>GPLGSISQNKRRYRKDGFDLDLTYVTDHVIAMSFPSSGRQSLFRNPIGEVSRFFKTKHPDK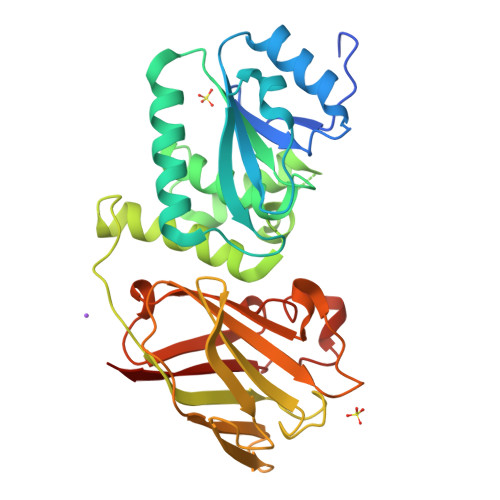FRIYNLCSERGYDETKFDNHVYRVMIDDHNVPTLVDLLKFIDDAKVWMTSDPDHVIAIHCKGGKGRTGTLVSSWLLEDGKFDTAKEALEYFGSRRTDFEVGDVFQGVETASQIRYVGYFEKIKKNYGGQLPPMKKLKVTGVTITAIQGVGRGNGSDLSMQIVSERQEVLLCKFAEGYNCALQYDATDDCVTCEVKNCPVLAGDIKVRFMSTSKSLPRGYDNCPFYFWFNTSLVEGDHVTLKREEIDNPHKKKTWKIYRDNFTVKLTFSDAEDI[3x]> HHHHHHMGSYGELIREIRLSKGLTQKEVYTGIISRSYAIGFEKGKHEITLSLFEEILKRIMVPLDEFFFIYRDFSSTEDDSFWIDFVELSGKNDVVGMQALLDKITLERTEQSEVRKAILHTRIQTINHYLRTNVFDESNISDEYKKIIHDYLWKMQTWTLEEVRIFSNGISFFEEEVQIHFYQIMLKSYEKYRYYDRGRLLFCHLFANLTDEL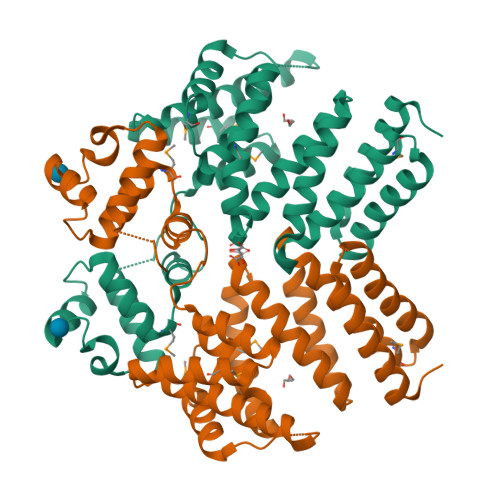IIQNKINYANLVLEKLKEASETSGSFNSAFYRIVANYYQGAIWMKEGEVEKGYRQAKRAIQTWKELHYEAIADLYSVVLKQFLEKENIQVED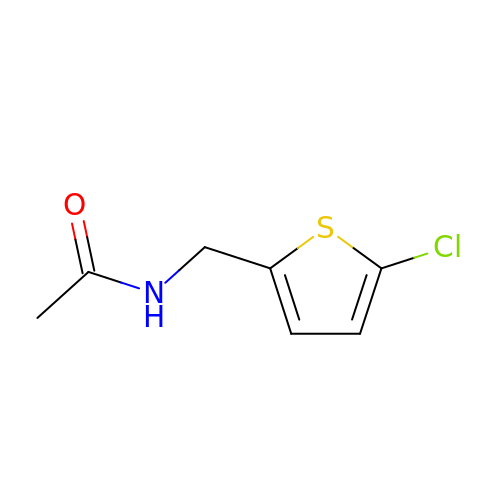N-[(5-chlorothiophen-2-yl)methyl]acetamide | C7 H8 Cl N O S | SYBYQBLOZYRNQY-UHFFFAOYSA-N The ice-nucleation protein InaZ from Pseudomonas syringae contains a large number of degenerate repeats that span more than a quarter of its sequence and include the segment GSTSTA. The ice-nucleation protein InaZ is produced by P. syringae and localized to its outer membrane. We chose to further investigate a segment whose sequence, GSTSTA, appears identically five times within InaZ at residues 707–712, 755–760, 803–808, 851–856 and 899–904. The benefits of racemic protein crystals for structure determination by MicroED were evaluated and it was confirmed that the phase restriction introduced by crystal centrosymmetry increases the number of successful trials during the ab initio phasing of the electron diffraction data. Both homochiral and racemic GSTSTA form amyloid-like protofibrils with labile, corrugated antiparallel β-sheets that mate face to back.

We optimized crystals of l-GSTSTA for microfocal X-ray diffraction, starting from dense needle clusters and ending with single needles. X-ray diffraction from a single crystal of l-GSTSTA yielded a 91.7% complete data set to approximately 1.1 Å resolution, while data sets from three crystals of l-GSTSTA obtained by MicroED were merged to achieve a data set with an overall completeness of 86.4% at 0.9 Å resolution. Atomic structure solutions were determined for l-GSTSTA from both microfocal X-ray and MicroED data by direct methods (Sheldrick, 2008). During refinement, the number of atoms in the X-ray structure increased to 36 peptide atoms and one bound water. The modeled water molecule also appears to be well ordered, particularly in the structure of l-GSTSTA determined by MicroED, where it has a B factor of 3.28 Å2. The single coordinated water is hydrogen-bonded to Ser708, the C-terminus of a symmetry-related strand and the backbone of Thr709 in the mating sheet. Homochiral GSTSTA forms a class 8 zipper in which two in-register, antiparallel β-sheets meet, related by a 180° rotation normal to the protofibril growth axis. Side chains between neighboring sheets tightly interdigitate to create a close packing within the fibril; the inter-sheet distances range from 5 to 7 Å. The l-GSTSTA protofibril appears tightly restrained within the crystal structure, as shown by a mean B factor of 0.92 Å2.

> GSTSTA> RTQSSTGTHGGYYYSFWTDNPNTVTYTNQNAGQFSVSWSGNQGNFVGGKGWNPGAARTIKYSGTYNPNGNSYLAVYGWTRNPLIEYYIVENFGTYNPSSGATAAGEVTVDGSVYDIYTSTRTNAPSIEGTRTFQQYWSVRRNKRSSGSVNTGAHFNAWSNVGLALGSHDYQILAVEGYYSSGSATMTVS

Serial crystallography at conventional synchrotron light sources (SSX) offers the possibility to routinely collect data at room temperature using micrometre-sized crystals of biological macromolecules. We show here the versatility of this setup and methodology by performing structural studies at room temperature (RT) of three additional enzyme systems of biological relevance: (i) Klebsiella pneumoniae CTX-M-14 β-lactamase, a β-lactamase relevant to multi-antibiotic resistance mechanisms; (ii) Nectria haematococca xylanase GH11, a highly active xylanase suitable for industrial applications; and (iii) Aspergillus flavus urate oxidase (UOX) in the presence of the long-lived intermediate-like 5-per­oxy-9-methyl-isourate (5PMUA).

In the case of N. haematococca xylanase (GH11) the crystal symmetry does not change with crystal size. The structural models resulting from refinement against the RT-SSX datasets are the first RT datasets of this N. haematococca xylanase. To inspect fluctuations in data quality and indexing rates, the run was split into 40 independent datasets, each consisting of 1000 detector images, and processed with the CrystFEL pipeline separately. Next, 1000, 2000, 3000, 4000, 5000, 6000, 8000, 10 000, 15 000, 20 000, 30 000 and finally all 40 000 detector images were processed together with partialator to assess the number of indexed images needed for a full dataset. Going from 1000 images to 40 000 images, the resolution at which CC* reaches 0.5 (the typical cut-off level in macromolecular crystallography) goes from 1.83 Å down to 1.5 Å [see Fig. 4(a)]. The alignment of all the residues of the active site (S19, W21, Y76, Y80, E89, Y91, P101, R125, Q139, Y174, E180 and Y182) is slightly worse, with an all-atom RMSD of 0.519 Å and comparable with the all-atom RMSD of all the residues (0.583 Å). The same alignment carried out using the 1000-image dataset, instead of the 40k dataset, resulted in a slightly worse all-atom RMSD of 0.630 Å. For just the two catalytic residues E89 and E180, the all-atom RMSD is 0.151 Å, overall the residues in the active site align very well in all three cases. At the same time, the TapeDrive system allows for uninterrupted data collection without manual intervention or the need to enter the hutch, enabling future automated multi-parameter data collection for multidimensional serial crystallography. This was demonstrated by collecting 40 datasets in less than 30 min, wherein each dataset had good statistics and usable diffraction to a resolution of better than 2 Å and each dataset took 40 s to collect with a PILATUS 6M detector, corresponding to only 7.5 s using an EIGER 16M (Dectris, Switzerland) at 133 Hz. If a higher resolution is desired, longer data collection times improve resolution, i.e. recording more indexable detector images, with a sweet spot, in this case, at roughly 4000 images.In this work, we exhaustively probe the ability of all 36 immobile HJ sequences to form DNA crystals in two different designed systems. Three separate self-assembling DNA crystal systems are described in this report: the “4 × 5” and “4 × 6” designs (collectively referred to as the 4 × N systems), and a third construct with a “scrambled” sequence variant of the 4 × 6 lattices. Self-assembly was mediated by three constituent oligonucleotides: (S1) containing four sequence repeats of either 5 or 6 bases; (S2) composed of 21 bases containing complementary regions to both (S1); and (S3) which forms the second junction crossover. The HJ serves as the fundamental component at the core of each unit, and the ultimate assembly of the full lattice is facilitated by the complementary 2-base sticky ends that tail each duplex.

We hypothesized that it might be possible to introduce other unique immobile sequences that could provide slight perturbations in the junction angle, to potentially reduce the strain in the original system and yield a “relaxed,” periodic lattice. The 4 × 5 system robustly crystallized with 75% of the junctions, and we obtained crystals in all but 9 of 36 sequences. Of the resulting structures, 18 exhibited P32 symmetry with average cell dimensions a = b = 68.85 Å c = 60.09 Å, with only nine retaining the original P3221 symmetry with average cell edges a = b = 68.17 Å c = 60.60 Å. Although the cell parameters between the two symmetries were virtually indistinguishable, the differences between the periodicity of the lattices is dramatic, with vastly different cavity sizes. We hypothesize that even a small difference in junction angles could have a significant global effect on the assembly of the lattice, thereby eliminating the strain in the P3221 lattices. However, in the majority of the crystal structures reported here, the cacodylate anion indeed fits best into the electron density map of our X-ray structures, due to the presence of sodium cacodylate in the crystallization solution.

> GAGCAGACATG;> ACTGCACTCA;> CAAGT;> TCTGAGTGCTGTCTGC> MGELRVGLEESELWLRFKELTNEMIVTKNGRRMFPVLKVNVSGLDPNAMYSFLLDFVAADNHRWKYVNGEWVPGGKPEPQAPSCVYIHPDSPNFGAHWMKAPVSFSKVKLTNKL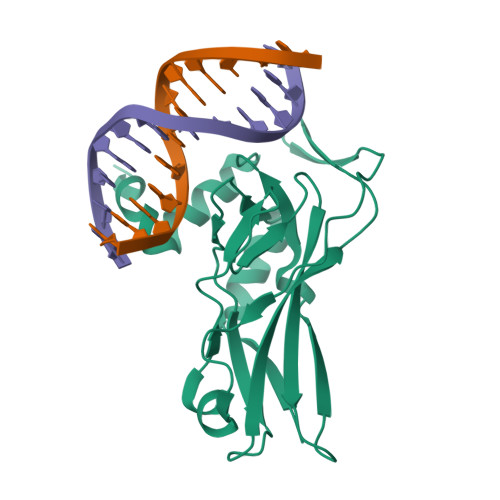NGGGQIMLNSLHKYEPRIHIVRVGGPQRMITSHCFPETQFIAVTAYQNEEITALKIKYNPFAKAFLDAKERSHHHHHH>LAKGLEDVYIDQTNICYIDGKEGKLYYRGYSVEELAELSTFEEVVYLLWWGKLPSLSELENFKKELAKSRGLPKEVIEIMEALPKNTHPMGALRTIISYLGNIDDSGDIPVTPEEVYRIGISVTAKIPTIVANWYRIKNGLEYVPPKEKLSHAANFLYMLHGEEPPKEWEKAMDVALILYAEHEINASTLAVMTVGSTLSDYYSAILAGIGALKGPIHGGAVEEAIKQFMEIGSPEKVEEWFFKALQQKRKIMGAGHRVYKTYDPRARIFKKYASKLGDKKLFEIAERLERLVEEYLSKKGISINVDYWSGLVFYGMKIPIELYTTIFAMGRIAGWTAHLAEYVSH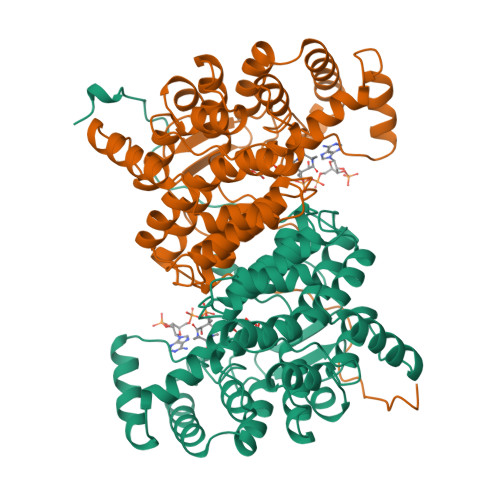NRIIRPRLQYVGEIGKKYLPIELRR[2x]> GPGSMMDEKMTDLTEEQKETLKKLKLYQKEYYDYESKFEYELFLLRQKYHDLYGPIYDKRREALVGNGEAKIGTPNLPEFWLRALRNNNTVSHVIEDHDEEILVYLNDIRCDYIKKNKEKKEGFILSFHFAPNPFFSNSVLTK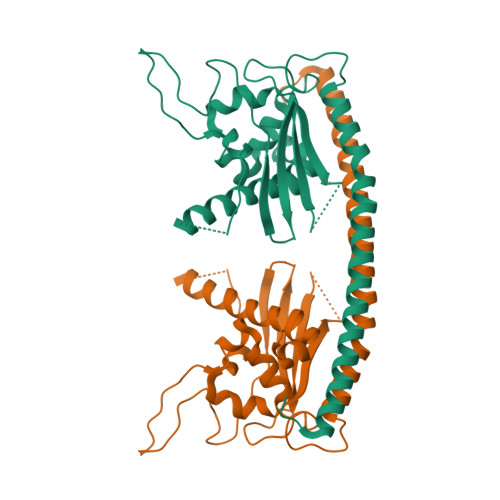TYHMKCVDCDNEPVLLHTEATVIDWYDNKNILKKNVVKKQHNKNSREVKTVQQTVNRDSFFHFFTSHKVPNSNVIKQLSKHEVAQLEMIIEGDYEVALTIKERIIPYAVDYFLGIIIESESNSIVSDVDSSYS>[3x]MRCIGISNRDFVEGVSSWVDIVLEHGSCVTTMAKNKPTLDFELIKTEAKQPATLRKYCIEAKLTNTTTESRCPTQGEPSLNEEQDKRFVCKHSMVDRGWGNGCGLFGKGGIVTCAMFRCKKNMEGKVVQPENLEYTVVITPHSGEEHAVGNDTGKHGKEVKITPQSSITEAELTGYGTVTMECSPRTGLDFNEMVLLQMENKAWLVHRQWFLDLPLPWLPGADTQGSNWIQKETLV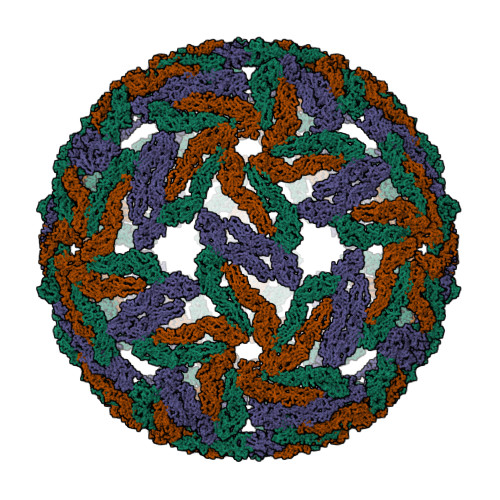TFKNPHAKKQDVVVLGSQEGAMHTALTGATEIQMSSGNLLFTGHLKCRLRMDKLQLKGMSYSMCTGKFKVVKEIAETQHGTIVIRVQYEGDGSPCKIPFEIMDLEKRHVLGRLITVNPIVTEKDSPVNIEAEPPFGDSYIIIGVEPGQLKLDWFKKG>MTQTTHHTPDTARQADPFPVKGMDAVVFAVGNAKQAAHYYSTAFGMQLVAYSGPENGSRETASYVLTNGSARFVLTSVIKPATPWGHFLADHVAEHGDGVVDLAIEVPDARAAHAYAIEHGARSVAEPYELKDEHGTVVLAAIATYGKTRHTLVDRTGYDGPYLPGYVAAAPIVEPPAHRTFQAIDHCVGNVELGRMNEWVGFYNKVMGFTNMKEFVGDDIATEYSALMSKVVADGTLKVKFPINEPALAKKKSQIDEYLEFYGGAGVQHIALNTGDIVETVRTMRAAGVQFLDTPDSYY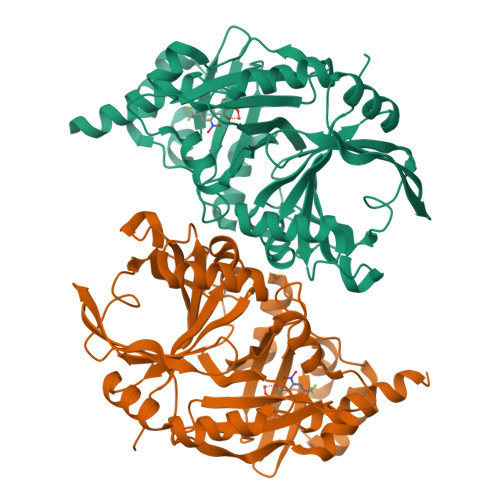DTLGEWVGDTRVPVDTLRELKILADRDEDGYLLQIFTKPVQDRPTVFFEIIERHGSMGFGKGNFKALFEAIEREQEKRGNL[2x]> MSLIYTITLNPAIDRLLFIRGELEKRKTNRVIKTEFDCGGKGLHVSGVLSKFGIKNEALGIAGSDNLDKLYAILKEKHINHDFLVEAGTSTRECFVVLSDDTNGSTMIPEAGFTVSQTNKDNLLKQIAKKVKKEDMVVIAGSPPPHYTLSDFKELLRTVKATGAFLGCDNSGEYLNLAVEMGVDFIKPNEDEVIAILDEKTNSLEENIRTLAEKIPYLVVSLGAKGSICAHNGKLYQVIPPKVQERNDTGAGDVFVGAFIAGLAMNMPITETLKVATGCS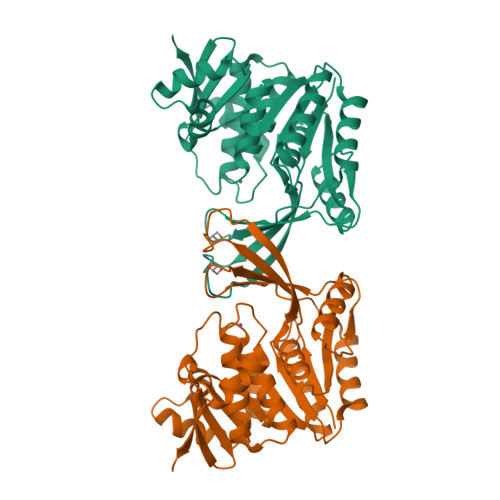ASAVMQQDSSSFDLEAAGKLKNQVSIIQLEEREGHHHHHH METHYL 3-{3-[(CYCLOHEXYLCARBONYL){[4'-(DIMETHYLAMINO)BIPHENYL-4-YL]METHYL}AMINO]PHENYL}ACRYLATE | C32 H38 N2 O3 | 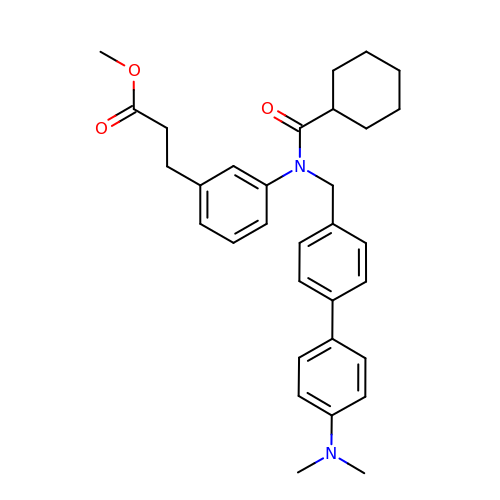GXGGBYHHVMOCJL-UHFFFAOYSA-N> ESEVEQTPLQEALNQLMRQLQR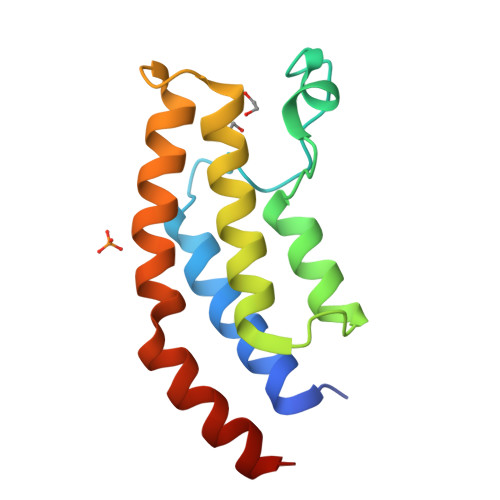KDPSAFFSFPVTDFIAPGYSMIIKHPMDFSTMKEKIKNNDYQSIEELKDNFKLMCTNAMIYNKPETIYYKAAKKLLHSGMKILSQERIQSLKQSIDFMADL>MERAMEQLNRLTRSLRRARTVELPEDNETAVYTLMPMVMADQHRSVSELLSNSKFDVNYAFGRVKRSLLHIAANCGSVECLVLLLKKGANPNYQDISGCTPLHLAARNGQKKCMSKLLEYSADVNICNNEGLTAIHWLAVNGRTELLHDLVQHVSDVDVEDAMGQTALHVACQNGHKTTVQCLLDSGADINRPNVSGATPLYFACSHGQRDTAQILLLRGAKYLPDKNGVTPLDLCVQGGYGETCEVLIQYHPRLFQTIIQMTQNEDLRENMLRQVLEHLSQQSESQYLKILTSLAEVATTNGHKLLSLSSNYDAQMKSLLRIVRMFCHVFRIGPSSPSNGIDMGYNGNKTPRSQVFKPLELLWHSLDEWLVLIATELMKNKRDSTEITSILLKQKGQDQDAASIPPFEPPGPGSYENLSTGTRESKPDALAGRQEASADCQDVISMTANRLSAVIQAFYMCCSCQMPPGMTSPRFIEFVCKHDEVLKCFVNRNPKIIFDHFHFLLECPELMSRFMHIIKAQPFKDRCEWFYEHLHSGQPDSDMVHRPVNENDILLVHRDSIFRSSCEVVSKANCAKLKQGIAVRFH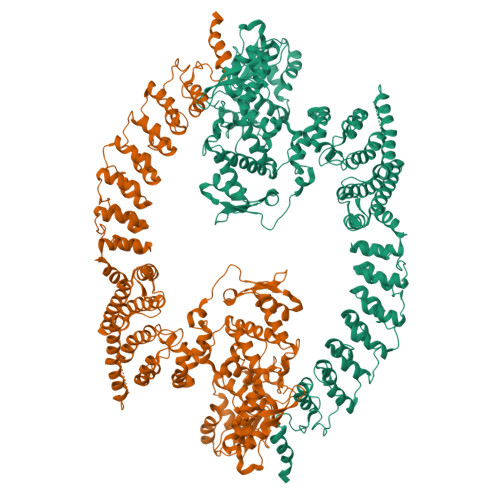GEEGMGQGVVREWFDILSNEIVNPDYALFTQSADGTTFQPNSNSYVNPDHLNYFRFAGQILGLALNHRQLVNIYFTRSFYKHILGIPVNYQDVASIDPEYAKNLQWILDNDISDLGLELTFSVETDVFGAMEEVPLKPGGGSILVTQNNKAEYVQLVTELRMTRAIQPQINAFLQGFHMFIPPSLIQLFDEYELELLLSGMPEIDVSDWIKNTEYTSGYEREDPVIQWFWEVVEDITQEERVLLLQFVTGSSRVPHGGFANIMGGSGLQNFTIAAVPYTPNLLPTSSTCINMLKLPEYPSKEILKDRLLVALHCGSYGYTMA[2x]>[2x]GAAUUGGGGGA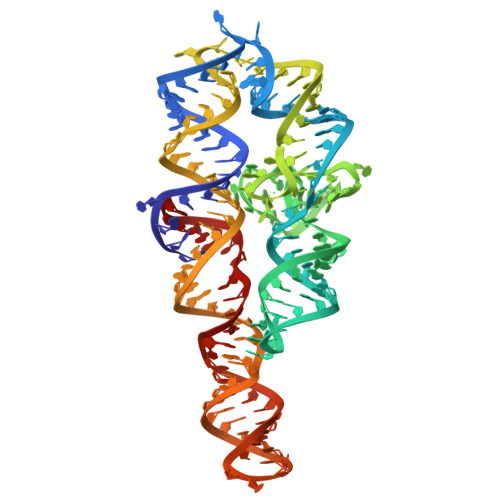AAGGGGUCAACAGCCGUUCAGUACCAAGUCUCAGGGGAAACUUUGAGAUGGCCUUGCAAAGGGUAUGGUAAUAAGCUGACGGACAUGGUCCUAACCCCCAGCCAAGUCCUAAGUCAACAGAUCUUCUGUUGAUAUGGAUGCAGUUC>[3x]MNVASRVVVNADRVKGTINRNIYGHFSEHLGRCIYEGLWVGEDSPIPNTNGIRNDVLEALKQMKIPVLHWPGGCFADEYHWKDGVGPREKRKRMVNTHWGGVIENNHFGTHEFMMLCELLGCEPYISGNVGSGTVQEMS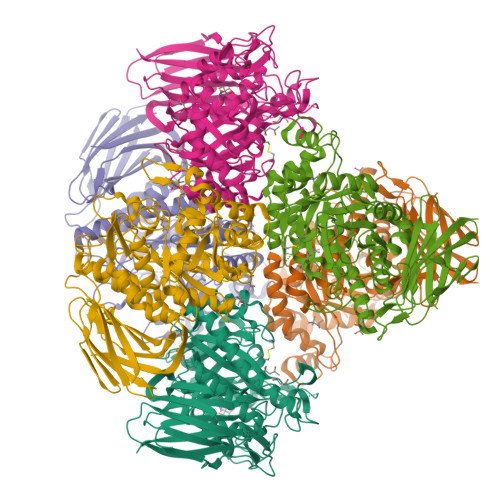EWVEYITFDGESPMANWRRENGREKPWRIKYWGVGNENWGCGGNMRAEYYADLYRQFQTYLRNYGDNKLHKIACGANTADYHWTEVLMKQAAPFMHGLSLHYYTVPGPWEKKGPATGFTTDEWWVTLKKALFMDELVTKHSAIMDVYDPDKRIDLIVDEWGTWYDVEPGTNPGFLYQQNSIRDALVAGATLHIFHRHCDRVRMANIAQLVNVMQSVILTEGERMLLTPTYHVFNMFKVHQDAELLDTWESVERTGPEGELPKVSVSASRAADGKIHISLCNLDFETGASVDIELRGLNGGVSATGTTLTSGRIDGHNTFDEPERVKPAPFRDFKLEGGHLNASLPPMSVTVLELTAG>MSQLELITSANQAFLEANPELTKLNKAPQRHIAIVTCMDTRLVNFAEDAIGVKRGEATVIKAAGNGIWTTGLSDIVVSLLVSIYELGVQEIFIMGHECCGMTHASTDSLGAQMLKSGIKPEDIEKFKSDLSKWVDDFKDPIDNIKNSVRCVRENPLIPKNIPIHGLLIHPDTGKVTTIINGY[2x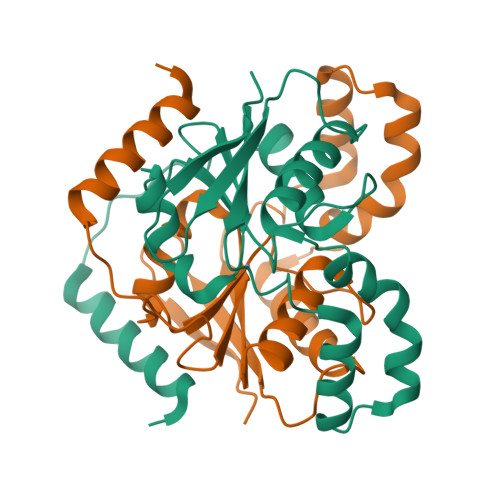]>[2x]GHMAEVLVVTSKVKKLIKEKGQMNTSAETIDVLSKAIEQLCLKGVESAKADGRKTVMARDIVIDHL

In this study, we present crystal structures and biochemical characterization of the free and DNA-bound forms of the histone homolog HBb from the predatory Gram-negative bacterium Bdellovibrio bacteriovorus. Our findings demonstrate that the single histone fold protein HBb forms a homodimer that has the ability to bind and bend DNA. Furthermore, we establish that HBb is essential for maintaining bacterial viability. Building on this, by employing various biophysical and biochemical approaches, we further substantiated the ability of HBb to bind and compact DNA by bending in a sequence-independent manner.

Similar to its free form, HBb successfully crystallized in complex with a randomized 20 bp DNA fragment (20 bp-GC50) within a few days, yielding the two distinct crystal forms HBb-DNA_1 and HBb-DNA_2. These could be processed to a resolution of 1.95 Å (HBb-DNA_1) and 1.85 Å (HBb-DNA_2), and solved by molecular replacement using the free form of HBb as a search model. In contrast, HBb-DNA_2 reveals a complementary DNA binding interface. Here, the asymmetric unit contains a 9 nucleotide (nt) long single-stranded DNA fragment, which forms dsDNA fragments via crystallographic symmetry. These fragments are bound by HBb via an additional interface of the minor groove. The crystal packing in HBb-DNA_2 markedly differs from that in HBb-DNA_1 in terms of the arrangement of the HBb dimers and DNA, containing only short DNA segments. The superposition of the HBb-DNA_1 and HBb-DNA_2 structures illustrates the location of the combined HBb-DNA binding interfaces, resembling histone-DNA complexes found in eukaryotes and archaea. The engagement of these interfaces suggests that the DNA undergoes bending upon binding with the HBb dimers.The membrane-anchored SNARE (soluble N-ethylmaleimide-sensitive factor acceptor protein receptor) proteins provide the energy to drive membrane fusion in various cellular contexts, such as intracellular trafficking and exocytosis. Supercomplexes of NSF, α-SNAP, and either a syntaxin tetramer or one of two binary complexes of syntaxin—SNAP-25 reveal atomic details of SNARE processing and show how sequential ATP hydrolysis drives disassembly. NSF comprises three structured domains connected by flexible linkers—the adapter N-domain followed by the D1 and D2 AAA+ domains. Six NSF protomers come together to form the active form of the enzyme, a homo-hexamer.

Furthermore, we were able to reproduce this result by reconstituting the complex with only the SNARE domains of syntaxin and SNAP-25 under non-hydrolyzing conditions (min22bin20S), yielding the same spire configuration but to a higher resolution of 3.86 Å following local reconstruction. This reconstruction also reveals the interface between an N-domain of NSF and an ɑ-SNAP molecule in detail; the interface is characterized by a core hydrophobic interaction surrounded by charge complementation. Four ɑ-SNAP molecules bind the 2:2 binary SNARE complex, with two SNAP-25 SN1 SNARE domains and two syntaxin H3 domains.

>[6x]GAHMAGRSMQAARCPTDELSLSNCAVVSEKDYQSGQHVIVRTSPNHKYIFTLRTHPSVVPGSVAFSLPQRKWAGLSIGQEIEVALYSFDKAKQCIGTMTIEIDFLQKKNIDSNPYDTDKMAAEFIQQFNNQAFSVGQQLVFSFNDKLFGLLVKDIEAMDPSILKGEPASGKRQKIEVGLVVGNSQVAFEKAENSSLNLIGKAKTKENRQSIINPDWNFEKMGIGGLDKEFSDIFRRAFASRVFPPEIVEQMGCKHVKGILLYGPPGCGKTLLARQIGKMLNAREPKVVNGPEILNKYVGESEANIRKLFADAEEEQRRLGANSGLHIIIFDEIDAICKQRGSMAGSTGVHDTVVNQLLSKIDGVEQLNNILVIGMTNRPDLIDEALLRPGRLEVKMEIGLPDEKGRLQILHIHTARMRGHQLLSADVDIKELAVETKNFSGAELEGLVRAAQSTAMNRHIKASTKVEVDMEKAESLQVTRGDFLASLENDIKPAFGTNQEDYASYIMNGIIKWGDPVTRVLDDGELLVQQTKNSDRTPLVSVLLEGPPHSGKTALAAKIAEESNFPFIKICSPDKMIGFSETAKCQAMKKIFDDAYKSQLSCVVVDDIERLLDYVPIGPRFSNLVLQALLVLLKKAPPQGRKLLIIGTTSRKDVLQEMEMLNAFSTTIHVPNIATGEQLLEALELLGNFKDKERTTIAQQVKGKKVWIGIKKLLMLIEMSLQMDPEYRVRKFLALLREEGASPLDFD;>SMAEDADMRNELEEMQRRADQLADESLESTRRMLQLVEESKDAGIRTLVMLDEQGEQLERIEEGMDQINKDMKEAEKNLTDLGK[2x];>MALSEIETRHSEIIKLENSIRELHDMFMDMAMLVESQGEMIDRIEYNVEHAVDYVERAVSDTKKAVKYQSKARRKKIM[2x];>[4x]GMDTSGKQAEAMALLAEAERKVKNSQSFFSGLFGGSSKIEEACEIYARAANMFKMAKNWSAAGNAFCQAAQLHLQLQSKHDAATCFVDAGNAFKKADPQEAINCLMRAIEIYTDMGRFTIAAKHHISIAEIYETELVDVEKAIAHYEQSADYYKGEESNSSANKCLLKVAGYAAQLEQYQKAIDIYEQVGTSAMDSPLLKYSAKDYFFKAALCHFCIDMLNAKLAVQKYEELFPAFSDSRECKLMKKLLEAHEEQNVDSYTESVKEYDSISRLDQWLTTMLLRIKKTIQGDEEDLR>AITSNEIGTHDGYDYEFWKDSGGSGSMTLNSGGTFSAQWSNVNNILFRKGKKFDETQTHQQIGNMSINYGATYNPNGNSYLAVYGWTVDPLVEFYIVDSWGTWRPPGGTPKGTINVDGGTYQIYETTRYNQPSIKGTATFQQYWSVRTSKRTSGTISVSEHFRAWESLGMNMGNMYEVALTVEGYQSSGSANVYSNTLTIGGQSGGEQATRVEAESMTKGGPYTSNITSPFNGVALYANGDNVSFNHSFTKANSSFSLRGASNNSNMARVDLRIGGQNRGTFYFGDQYPAVYTINNINHGIGNQLVELIVTADDGTWDA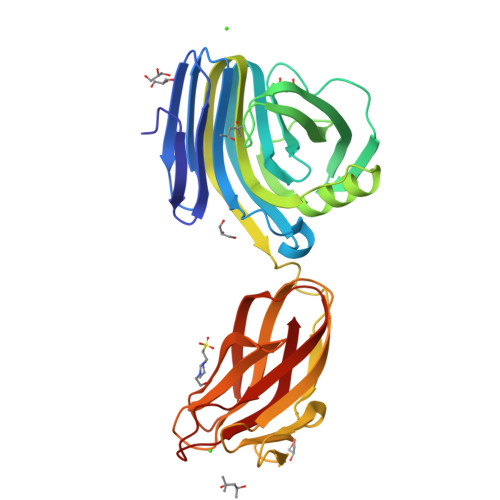YLDYLEIR[2x]> SVVELGKMIIQETGKSPFPSYTSYGCFCGGGERGPPLDATDRCCLAHSCCYDTLPDCS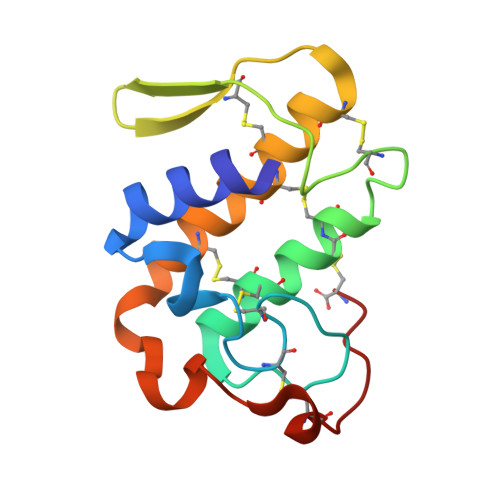PKTDRYKYKRENGEIICENSTSCKKRICECDKAVAVCLRKNLNTYNKKYTYYPNFWCKGDIEKC> DPDQFRAIIESPEGAGHVGYQYRRNTGSTMRMVSDVLDERVSLWDFHCDPSGNVIQPGPNVDSRQYLQAAI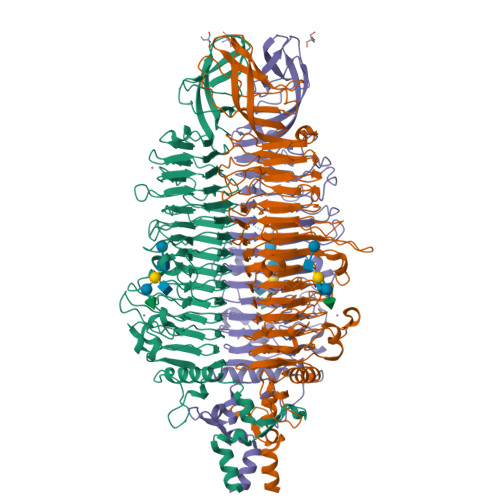DYVSSNGGGTITIPAGYTWYLGSYGVGGIAGHSGIIQLRSNVNLNIEGRIHLSPFFDLKPFQVFVGFDNGDPASSGNLENCHIYGHGVVDFGGYEFGASSQLRNGVAFGRSYNCSVTGITFQNGDVTWAITLGWNGYGSNCYVRKCRFINLVNSSVNADHSTVYVNCPYSGVESCYFSMSSSFARNIACSVQLHQHDTFYRGSTVNGYCRGAYVVMHAAEAAGAGSYAYNMQVENNIAVIYGQFVILGSDVTATVSGHLNDVIVSGNIVSIGERAAFSAPFGAFIDIGPDGASNVQDIQRVLVTGNSFYAPANITDSAAITLRANLNGCTFIANNFDCRYMVYNAPGTTSPVVQNLVWDKSNVIGGTHANQRAGQNLFDMQFASVVNSTIEVQLSCEDLSMFSCILFPASCQLSYSKITVDSAWTKSMSNTAVFEGNQQAGANVYVSYPATVNLTSYNTQGAVPFFSTDTNYAWVTSAYSLSINENLDFSPPATYTNKANGQLVGVGYNEIGGVRSVSVRLMLQRQV>[2x]MSATKSIVGEALEYVNIGLSHFLALPLAQRISLIIIIPFIYNIVWQLLYSLRKDRPPLVFYWIPWVGSAVVYGMKPYEFFEECQKKYGDIFSFVLLGRVMTVYLGPKGHEFVFNAKLADVSAEAAYAHLTTPVFGKGVIYDCPNSRLMEQKKFVKGALTKEAFKSYVPLIAEEVYKYFRDSKNFRLNERTTGTIDVMVTQPEMTIFTASRSLLGKEMRAKLDTDFAYLYSDLDKGFTPINFVFPNLPLEHYRKRDHAQKAISGTYMSLIKERRKNNDIQDRDLIDSLMKNSTYKDGVKMTDQEIANLLIGVLMGGQHTSAATSAWILLHLAERPDVQQELYEEQMRVLDGGKKELTYDLLQEMPLLNQTIKETLRMHHPLHSLFRKVMKDMHVPNTSYAIPAGYHVLVSPGYTHLRDEYFPNAHQFNIHRWNNDSASSYSVGEEVDYGFGAISKGVSSPYLPFGGGRHRCIGEHFAYCQLGVLMSIFIRTLKWHYPEGKTVPPPDFTSMVTLPTGPAKIIWEKRNPEQKIGGRHHHHHH

Lanosterol 14α-demethylase (CYP51 or Erg11p in yeast and some fungal pathogens; sterol 14α-demethylase in fungal phytopathogens) is the primary target of the imidazole and triazole (azole) antifungal drugs, often referred to as demethylase inhibitors (DMIs). The CYP51 enzymes of fungal pathogens and yeast use eburicol or lanosterol as substrates to produce ergosterol while their orthologues in plants and humans use obtusifoliol and lanosterol, respectively, to produce plant sterols and cholesterol. In order to better understanding the activity of DMI agrochemicals, we have determined how selected antifungals interact with their target enzyme using S. cerevisiae lanosterol 14α-demethylase as a surrogate. We have also determined seven high resolution X-ray crystal structures of ScErg11p6×His in complex with R- and S-TBZ, R- and S-DPZ, FQZ, PRZ and DFC.

FQZ binds unambiguously in the active site via a coordinate bond between the N3 of the triazole ring and the iron of the heme cofactor. The dichlorophenyl ring binds deep in the active site adjacent to G310 in a similar manner to FLC. The rigid quinazolin-4(3H)-one ring projects towards the entry channel in an orientation with the aromatic ring perpendicular to the non-coordinating azole of FLC. Y126 is shifted away compared to the FLC structure to accommodate the rigid and bulky ring system with a close contact between the fluoro substituent of the fungicide and the phenolic ring. No water (743/843) is seen adjacent to Y140. A limited number of water molecules were modelled into the structure of ScErg11p6×His in complex with FQZ due to the relatively low resolution of this structure. All complexes were crystallised in the space group P 1 211, with a single ScErg11p6×His-ligand complex in the asymmetric unit, with the exception of the ScErg11p6×His -FQZ complex, which was crystallised in space group P1 with two protomers found in the asymmetric unit. Comparison of the ScErg11p6×His-FQZ complex with the others shows an almost identical protein structure, including the transmembrane and amphipathic helices. There are two protomers in the asymmetric unit and the interface between the two protomers includes direct hydrogen bonding interactions between the phenolic hydroxyl of Y341 and the main chain carbonyl oxygen of E418’ with a salt bridge between E342 and K107’. Again we observed 8.3 fold (3.3 ± 0.7 μM) and 4 fold (1.6 ± 0.5 μM) reduction in susceptibility to FQZ in the Y140F and Y140H mutant strains respectively.>DRHHHHHHKLQHVPPWTEDCRKSTYPPSGPTYRGPVPWYTINLDLPPYKRWHELMVDKAPALKVIVNYLKNMINAFEPSGKIVQLVDQKLPGLLGSFPGPFEEEMKGIAAVTEIPLGEIILFNIFYEFFTIATSIITEDKEGHLLHARNMDFGVFLGWNVNNNTWVVTEELKPLTVNLDFQRNSKTVFKAAGFAGYVGMLTGFKPGLFSLTLNERFSTNGGFMGVIEWILGKKDAKWIGFIIRSVLENSTSYEEAKTILTKSKILAPAYFILGGSKSGEGCVITRDRVQSLDIYELDPKQGI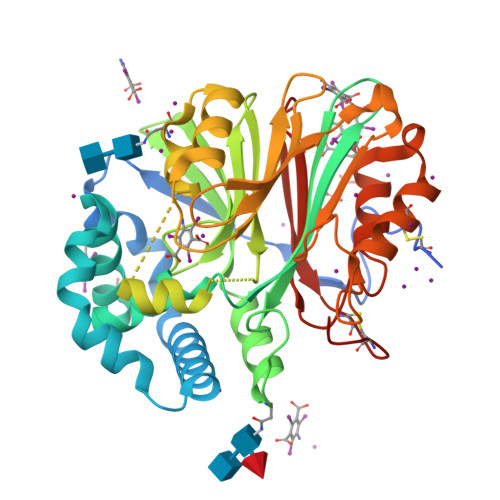WYVVQTNYDRWKNPFFLDNRRTPAKMCLNRTTQENISFATMYDVLSTKPVLNKLTVYTALIDVTKGQFETYLRDCPDPCIGW[2x]>SRPLSDQEKRKQISVRGLAGVENVTELKKNFNRHLHFTLVKDRNVATPRDYYFALAHTVRDHLVGRWIRTQQHYYEKDPKRIYYLSLEFYMGRTLQNTMVNLALENACDEATYQLGLDMEELEEIEEDAGLGNGGLGRLAACFLDSMATLGLAAYGYGIRYEFGIFNQKICGGWQMEEADDWLRYGNPWEKARPEFTLPVHFYGRVEHTSQGAKWVDTQVVLAMPYDTPVPGYRNNVVNTMRLWSAKAPNDFNLKDFNVGGYIQAVLDRNLAENISRVLYPNDNFFEGKELRLKQEYFVVAATLQDIIRRFKSSKFGCRDPVRTNFDAFPDKVAIQLNDTHPSLAIPELMRVLVDLERLDWDKAWEVTVKTCAYTNHTVIPEALERWPVHLLETLLPRHLQIIYEINQRFLNRVAAAFPGDVDRLRRMSLVEEGAVKRINMAHLCIAGSHAVNGVARIHSEILKKTIFKDFYELEPHKFQNKTNGITPRRWLVLCNPGLAEIIAERIGEEYISDLDQLRKLLSYVDDEAFIRDVAKVKQENKLKFAAYLEREYKVHINPNSLFDVQVKRIHEYKRQLLNCLHVITLYNRIKKEPNKFVVPRTVMIGGKAAPGYHMAKMIIKLITAIGDVVNHDPVVGDRLRVIFLENYRVSLAEKVIPAADLSEQISTAGTEASGTGNMKFMLNGALTIGTMDGANVEMAEEAGEENFFIFGMRVEDVDRLDQRGYNAQEYYDRIPELRQIIEQLSSGFFSPKQPDLFKD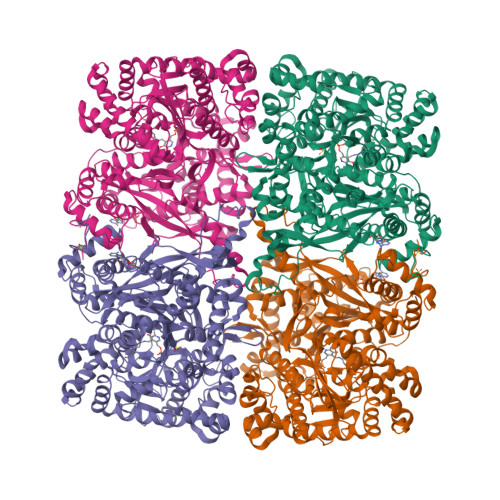IVNMLMHHDRFKVFADYEEYVKCQERVSALYKNPREWTRMVIRNIATSGKFSSDRTIAQYAREIWGVEPSRQRLPAPDEKIP[4x]>MNSTPKGTIYLTFSDGPVNASVEVIKVLNQGGVKATFYFNAWHLDGIGDENEDRALEALKLALDSGHIVGNHSYDHMIHNCVEEFGPTSGADCNATGNHQIHSYQDPVRDAASFEQNLITLEKYLPTIRSYPNYKGYELARLPYTNGWRVTKHFQADGLCATSDNLKPWEPGYVCDPANPSNSVKASIQVQNILANQGYQTHGWDVDWAPENWGIPMPANSLTEAVPFLAYVDKALNSCSPTTIEPINSKTQEFPCGTPLHADKVIVLTHDFLFEDGKRGMGATQNLPKLAEFIRIAKEAGYVFDTMDNYTPRWSVGKTYQAGEYVLYQGVVYKAVISHTAQQDWAPSSTSSLWTNADPATNWTLNVSYEQGDIVNYKGKRYLVSVPHVSQQDWTPDTQNTLFTALELR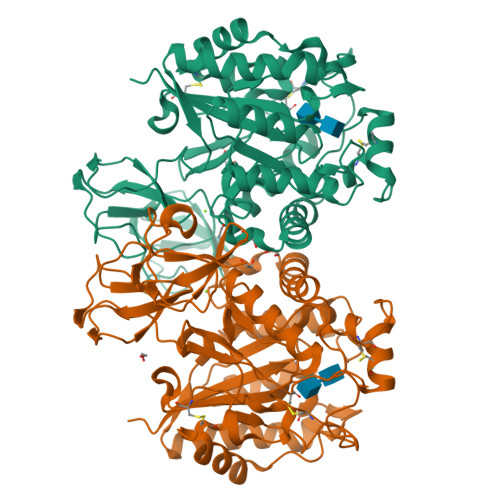RQWSHPQFEK[2x]>[2x]GPGSPGPPEHVRVDEITDTTAQISWQEGTDNHSPVTAYTIQARTPFSVGWQRVTTVPDVIDGNTFTTTVVDLNPWVEYEFRVVASNKIGGGEPSLPSEKVRTEEAVPEIPPAEVSGGGGSRSELVITWDPIPEELQNGEGFGYVVAFRPFGTTTWIQTVVTSPDTPRYVFRNESILPFSPYEVKVGVYNNKGEGPFSSITTVFSAEGGGSG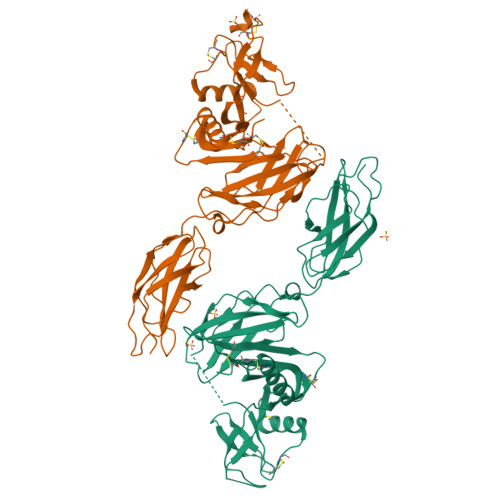GGSEVPADGNAGLLAEPQIAMFCGKLNMHMNVQNGKWESDPSGTKTCIDTKEGILQYCQEVYPELQITNVVEANQPVTIQNWCKRGWKQCNGHPHIVVPYRCLVGEFVSDALLVPDKCKLLHQERMDVCETHLHWHTVAKESCSEKSMNLHDYGMLLPCGIDKFRGVEFVCCPLAEESDNLDSAAA> GMQEHYQPAAIEPAAQKKWDDARISNVSEDASKPKYYCLSMFPYPSGKLHMGHVRNYTIGDVLSRFKLLNGFNVMQPMGWDAFGMPAENAAMKNNVAPAAWTYDNIEYMKTQLKSLGFAVDWEREVATCKPEYYRWEQWLFTKLFEKGIVYRKNGTVNWDPVDQTVLANEQVIDGRGWRSGALIEKREIPMYYFKITDYAEELLNDLDKLEHWPEQVKTMQRNWIGKSRGMTVRFAVSDDSKQGLEGDYAKFLQVYTTRPDTLMGATYVAVAAEHPLATAAAADKPELQAFIAECKAGSVAEADMATMEKKGVPTGRYVVNPLNGDKLEVWIANYVLWGYGDGAVMAVPAHDERDFEFAAKYNLPKKQVIAVGDNAFDANRWQEWYGDKENGVLVNSGDLDGLDFQTAFDAVAAKLQSQGAGEPKTQYRLRDWGISRQRYWGCPIPIVHCEKCGNVPVPADQLPVVLPENVVPDGMGSPLAKMPEFYETSCPCCGGAAKRETDTMDT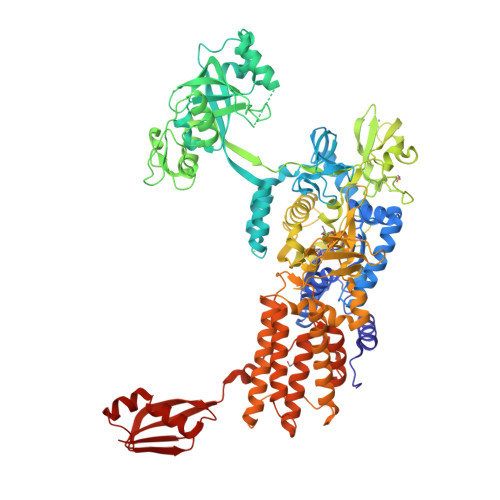FIESSWYFFRYMSPKFSDGMVSAESAKYWGAVDQYIGGIEHAIAHLLYARFFTKLMRDEGLVNVDEPFERLLTQGMVVCETYYRENDKGGKDWINPADVELTFDDKGRPVSAVLKADGLPVVISGTEKMSKSKNNGVDPQELINAYGADTARLFMMFAAPPEQSLEWSDSGVEGAHRFLRRLWRTVYEYLKQGGAVKAFAGNQDGLSKELKDLRHKLHSTTAKVSDDYGRRQQFNTAIAAVMELLNQYDKTDTGSEQGRAVAQEVLEAAVRLLWPIVPHICETLWSELNGAKLWEAGWPTVDEAALVKSEIEVMVQVNGKLRGKITVAADASKADLEAAALANEGAVKFMEGKPAKKIIVVPGRLVNIVV Clamp loaders are pentameric ATPases that place circular sliding clamps onto DNA, where they function in DNA replication and genome integrity. Because the sliding clamp is a closed ring in solution, it needs to be opened and placed onto DNA by a separate ATPase complex called the clamp loader. All clamp loaders are pentameric ATPases of the AAA + family (ATPases associated with various cellular activities). Here we describe a series of structures of the E. coli clamp loader in the process of placing the clamp onto a p/t-junction.

In the presence of ATPγS, we obtained an ∼8 Å resolution reconstruction of the clamp loader bound to a closed clamp. Despite the modest resolution of the reconstruction, we can unambiguously identify the location and orientation of all the protein domains of both the clamp loader and sliding clamp. We observe that the γ-complex contacts the sliding clamp primarily through the A, D, and E subunits; the B and C subunits make minimal contact with the surface of the clamp. Furthermore, the AAA+ modules of the B and C subunits make minimal contact with each other. As inter-subunit contacts are necessary to hydrolyze ATP, this separation between subunits likely inhibits ATPase activity. Because the clamp is closed in this state, we attribute this conformation as the initial-binding complex. The Initial-Binding state contains ATPγS, all other states contain ADP·BeFx. Despite the low resolution of the structure, we unambiguously observe that the γ-complex initially binds to a closed ß-clamp. The existence of a closed binding complex was predicted based on rapid kinetics studies which showed that clamp binding occurs before clamp opening. The γ-complex binds the ß-clamp using the A, D, and E subunits, and with the A-gate of the γ-complex open.

> MIRLYPEQLRAQLNEGLRAAYLLLGNDPLLLQESQDAVRQVAAAQGFEEHHTFSIDPNTDWNAIFSLCQAMSLFASRQTLLLLLPENGPNAAINEQLLTLTGLLHDDLLLIVRGNKLSKAQENAAWFTALANRSVQVTCQTPEQAQLPRWVAARAKQLNLELDDAANQVLCYCYEGNLLALAQALERLSLLWPDGKLTLPRVEQAVNDAAHFTPFHWVDALLMGKSKRALHILQQLRLEGSEPVILLRTLQRELLLLVNLKRQSAHTPLRALFDKHRVWQNRRGMMGEALNRLSQTQLRQAVQLLTRTELTLKQDYGQSVWAELEGLSLLLCHKPLADVFIDG;>[3x]GPHMSYQVLARKWRPQTFADVVGQEHVLTALANGLSLGRIHHAYLFSGTRGVGKTSIARLLAKGLNCETGITATPCGVCDNCREIEQGRFVDLIEIDAASRTKVEDTRDLLDNVQYAPARGRFKVYLIDEVHMLSRHSFNALLKTLEEPPEHVKFLLATTDPQKLPVTILSRCLQFHLKALDVEQIRHQLEHILNEEHIAHEPRALQLLARAAEGSLRDALSLTDQAIASGDGQVSTQAVSAMLGTLDDDQALSLVEAMVEANGERVMALINEAAARGIEWEALLVEMLGLLHRIAMVQLSPAALGNDMAAIELRMRELARTIPPTDIQLYYQTLLIGRKELPYAPDRRMGVEMTLLRALAFHPRMPLPEPEVPRQ;> GPHMRWYPWLRPDFEKLVASYQAGRGHHALLIQALPGMGDDALIYALSRYLLCQQPQGHKSCGHCRGCQLMQAGTHPDYYTLAPEKGKNTLGVDAVREVTEKLNEHARLGGAKVVWVTDAALLTDAAANALLKTLEEPPAETWFFLATREPERLLATLRSRCRLHYLAPPPEQYAVTWLSREVTMSQDALLAALRLSAGSPGAALALFQGDNWQARETLCQALAYSVPSGDWYSLLAALNHEQAPARLHWLATLLMDALKRHHGAAQVTNVDVPGLVAELANHLSPSRLQAILGDVCHIREQLMSVTGINRELLITDLLLRIEHYLQPGVVLPVPHL;>[2x]GPHMKFTVEREHLLKPLQQVSGPLGGRPTLPILGNLLLQVADGTLSLTGTDLEMEMVARVALVQPHEPGATTVPARKFFDICRGLPEGAEIAVQLEGERMLVRSGRSRFSLSTLPAADFPNLDDWQSEVEFTLPQATMKRLIEATQFSMAHQDVRYYLNGMLFETEGEELRTVATDGHRLAVCSMPIGQSLPSHSVIVPRKGVIELMRMLDGGDNPLRVQIGSNNIRAHVGDFIFTSKLVDGRFPDYRRVLPKNPDKHLEAGCDLLKQAFARAAILSNEKFRGVRLYVSENQLKITANNPEQEEAEEILDVTYSGAEMEIGFNVSYVLDVLNALKCENVRMMLTDSVSSVQIEDAASQSAAYVVMPMRL> MRRRSRMLLCFAFLWVLGIAYYMYSGGGSALAGGAGGGAGRKEDWNEIDPIKKKDLHHSNGEEKAQSMETLPPGKVRWPDFNQEAYVGGTMVRSGQDPYARNKFNQVESDKLRMDRAIPDTRHDQCQRKQWRVDLPATSVVITFHNEARSALLRTVVSVLKKSPPHLIKEIILVDDYSNDPEDGALLGKIEKVRVLRNDRREGLMRSRVRGADAAQAKVLTFLDSHCECNEHWLEPLLERVAEDRTRVVSPIIDVINMDNFQYVGASADLKGGFDWNLVFKWDYMTPEQRRSRQGNPVAPIKTPMIAGGLFVMDKFYFEELGKYDMMMDVWGGENLEISFRVWQCGGSLEIIPCSRVGHVFRKQHPYTFPGGSGTVFARNTRRAAEVWMDEYKNFYYAAVPSARNVPYGNIQSRLELRKKLSCKPFKWYLENVYPELRVPDHQDIAFGALQQGTNCLDTLGHFADGVVGVYECHNAGGNQEWALTKEKSVKHMDLCLTVVDRAPGSLIKLQGCREDDSRQKWEQIEGNSKLRHVGSN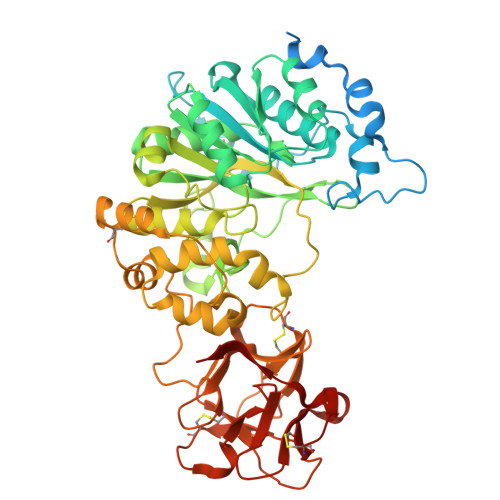LCLDSRTAKSGGLSVEVCGPALSQQWKFTLNLQQ>[2x]GIREVILCKDQDGKIGLRLKSVDNGIFVQLVQANSPASLVGLRFGDQVLQI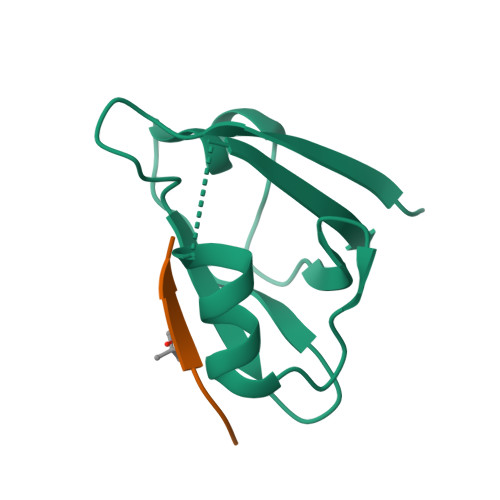NGENCAGWSSDKAHKVLKQAFGEKITMTIR;>[2x]SHWVXDI>GSSLRGGHAGTTYIFSKGGGQITYKWPPNDRPSTRADRLAIGFSTVQKEAVLVRVDSSSGLGDYLELHIHQGKIGVKFNVGTDDIAIEESNAIINDGKYHVVRFTRSGGNATLQVDSWPVIERYPAGNNDNERLAIARQRIPYRLGRVVDEWLLDKGRQLTIFNSQATIIIGGKEQGQPFQGQLSGLYYNGLKVLNMAAENDANIAIVGNVRLVG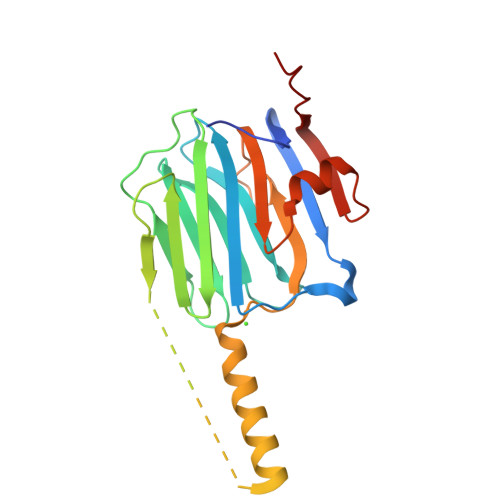EVPSS[2x]>GAMVVSPAGADRRIPTWASRVVSGLARDRPVVVTKEDLTQRLTEAGCGRDPDSAIRELRRIGWLVQLPVKGTWAFIPPGEAAISDPYLPLRSWLARDQNAGFMLAGASAAWHLGYLDRQPDGRIPI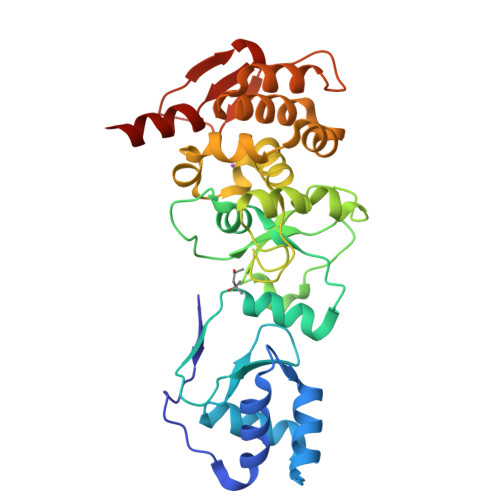WLPPAKRLPDGLASYVSVVRIPWNAADTALLAPRPALLVRRRLDLVAWATGLPALGPEALLVQIATRPASFGPWADLVPHLDDLVADCSDERLERLLSGRPTSAWQRASYLLDSGGEPARGQALLAKRHTEVMPVTRFTTAHSRDRGESVWAPEYQLVDELVVPLLRVIGKA[2x]The Myxococcus xanthus FrzS protein transits from pole-to-pole within the cell, accumulating at the pole that defines the direction of movement in social (S) motility. The N-terminal receiver domain (RD), a 258-residue coiled-coil domain, and the extreme C-terminal tail of the protein are all required for the dynamic subcellular localization and S-motility activity of FrzS. Here we show using atomic-resolution crystallography and NMR that the FrzS receiver domain (RD) displays the conserved switch Tyr102 in an unusual conformation, lacks the conserved Asp phosphorylation site, and fails to bind Mg2+ or the phosphoryl analogue, Mg2+·BeF3. The crystal structures of the mutants suggested that the observed conformation of Tyr102 in the wild-type FrzS RD is not sufficient for function. These results support the model that FrzS contains a novel ‘pseudo-receiver domain’ whose function requires recognition of the RD output face but not Asp phosphorylation.

To explore the potential for intramolecular signalling, we determined the crystal structure of the FrzS RD in two crystal forms, a hexagonal form (P63) at 1.0 Å resolution and a tetragonal form (I4) at 1.9 Å. After several rounds of refinement using data to 1.0 Å resolution, this structure was used to solve the tetragonal form. The FrzS RD structures in the two crystal forms were very similar, but the overall Cα RMSD for the structures of 0.57 Å was above the errors in the coordinates. The largest differences between the structures in the two crystal forms occurred in the conformation of the β3-α3 loop, part of which was modelled in two conformations in the hexagonal structure. Excluding these residues (54–62) from the comparison reduced the Cα RMSD to 0.45 Å. The tetragonal crystals contained three molecules in the asymmetric unit, one of which forms one side of a large solvent channel in the crystal lattice. Although the backbone conformation was very similar, this molecule was poorly ordered in the present structure, and virtually missing from the electron density when different cryoprotectants were used (N. Echols and J. Fraser, data not shown). Nonetheless, the independent structures in the tetragonal form provide an important control for the effects of crystal packing on the overall conformation. Even in the relatively unconstrained tetragonal crystal form, FrzS adopted approximately the same structure observed in the high-resolution crystals. The crystal contacts along the α4-β5-α5 face varied in the four independent molecules in the two crystal forms, suggesting that the similar side chain positions of critical residues, including Tyr102, faithfully represent the predominant conformation of the RD.

>[3x]GSHMSKKILIVESDTALSATLRSALEGRGFTVDETTDGKGSVEQIRRDRPDLVVLAVDLSAGQNGYLICGKLKKDDDLKNVPIVIIGNPDGFAQHRKLKAHADEYVAKPVDADQLVERAGALIGFPE> SNAMATHSTNE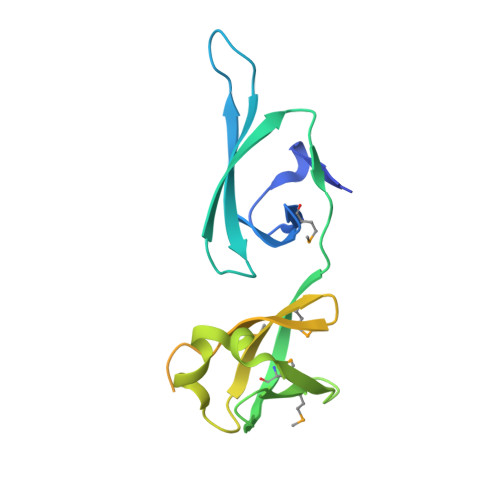FRGGLKVMVDGDPCSIIDNEFVKPGKGQAFNRVKFRNLKTGRVLERTFKSGETLPAADVVEVEMQYLYNDGEFWHFMTSENYEQHAASKEAVAEAKQWLKEEALCMVTMWNGVPLSVEPPNFVELKITETEPGVRGDTATGGTKRAKLETGAVVRVPLFLNEGEIIKVDTRRGEYVSRAK>[4x]MNHFDTIIIGGGPAGMMATISSSFYGQKTLLLEKNKRLGKKLAGTGGGRCNVTNNGNLDDLMAGIPGNGRFLYSVFSQFDNHDIINFFTENGVKLKVEDHGRVFPVTDKSRTIIEALEKKIAELGGTVITNTEIVSVKKTDELFTVRSSDQAWTCQKLIVTTGGKSYPSTGSTGFGHDIARHFKHTVTDLEAAESPLLTDFPHKALQGISLDDVTLSYGKHIITHDLL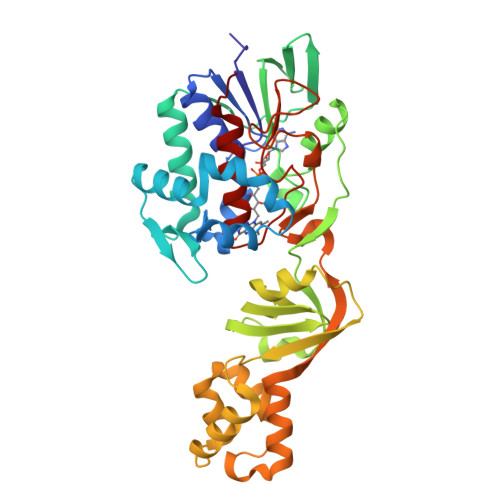FTHFGLSGPAALRLSSFVKGGETIYLDVLPQMSQQDLADFLEEHREKSLKNCLKILLPERIADFFTQPFPEKVKQLNLSEKEALIKQIKELPISVTGKMSLAKSFVTKGGVSLKEINPKTLESKLVPGLHFAGEVLDINAHTGGFNITSALCTGWVAGSLHYD>[2x]MAHHHHHHVDDDDKMLLPETRNLLDLMDAATRGGRPGLDTLPHAVGRKAVDKMSEDGEADPPEV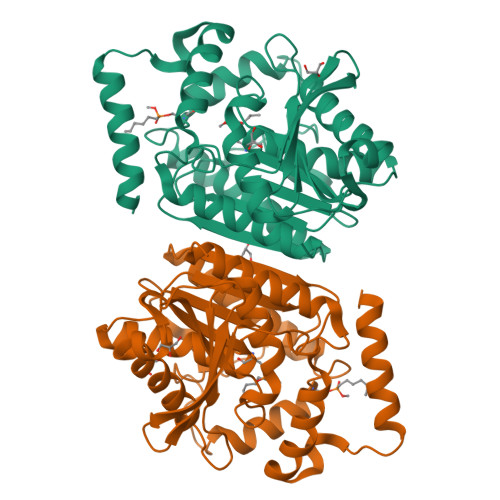AEVANGGFAGPASEIRFRRYRPLGEAAGLLPTLIYYHGGGFVIGNIETHDSTCRRLANKSRCQVISIDYRLAPEHPFPAPIDDGIAAFRHIRDNAESFGADAARLAVGGDSAGGAMAAVVCQACRDAGETGPAFQMLIYPATDSSRESASRVAFAEGYFLSKAHMDWFWEAYVPEDTDLTDLRLSPLLATDFTGLPPAFVLTAGYDPLRDEGRAYADRLIEAGIKTTYVNYPGTIHGFFSLTRFLSQGLKANDEAAAVMGAHFGT Type I-D CRISPR–Cas systems, which are found both in bacteria and archaea, are exceptional in that they contain a hybrid large subunit, Cas10d, bearing resemblance to both the signature proteins found in type I (Cas3) and type III (Cas10). Here, we present the crystal structure of the Cas10d large effector complex subunit from the Sulfolobus islandicus I-D system, both in isolation and in complex with the Sulfolobus islandicus rod-shaped virus 3 (SIRV3) anti-CRISPR protein, AcrID1. As predicted from comparative sequence analysis, the 847 residue (94 kDa) S. islandicus Cas10d consists of six domains: A HD nuclease domain (1–186), a Cyclase/RRM domain (187–425), a zinc finger domain (426–490), a Palm/RRM domain (491–623), and a C-terminal helical region consisting of a polymerase-like Thumb domain (624–719) and an extension with predicted homology to Cas11 (720–847). In this paper, we demonstrate that the S. islandicus type I-D large subunit, Cas10d, has a unique structure consisting of a type I-like HD nuclease domain joined to a set of inactivated type III-like nucleotidyl transferase domains and a Cas11-like C-terminal domain.

To answer this, we finally pursued a structure of the isolated Cas10d subunit. The isolated protein does not readily crystallise likely due to intrinsic flexibility, however, we were able to obtain crystals of a mildly trypsin-treated sample and determine the structure at 4.0 Å using molecular replacement. The new crystals contain two copies of Cas10d in the crystallographic asymmetric unit, for which the flexible N terminus (residues 1–13) that interacts with AcrID1, appears to have been cleaved off. Moreover, the Palm/RRM domain has been nicked by the protease resulting in the protein appearing as two bands on a denaturing polyacrylamide gel. Nevertheless, the structure confirms the overall, extended conformation of Cas10d as observed in complex with AcrID1. The helical insertion in the Palm/RRM domain, which interacts directly with AcrID1 in the complex structure, has shifted away from the core of the protein by about 5 Å in comparison to the complex with AcrID1. Together, this suggests that the flexibility of Cas10d is mainly caused by the extended Palm/RRM domain. Consequently, it is likely that this domain gets organised when Cas10d joins the backbone complex and forms the complete I-D effector complex. In summary, we conclude that the extended structure of Cas10d is an intrinsic feature and not an effect of AcrID1 binding.

>MRNLKRIVMGENKLIGLVRTALDSITLGQGVNEAKIKSPQSYAFHTISVGTISLDICKAIYSSSEIGRKQLENLSKKYNMPFEDLWFYGGFLHDWNKLSGKEESLENKEELTKKIIDKLKLPNEFLHGISTMAEGHLPDNLHLPLWVSIKLADMLLISDIGSVRDVFYFANSDSYRNAIEALKEYNLELNYVSSTFRLFTLIASKELLNDVFNEKSGYFPLISYADGIVFLKRKNSQPVLLSKIVDLLSRQVFSSSSEVIEEKISDIEKCIKNKEELFRQMNIDVKSAIYDEEGKVKQINAFLPTKVCKPFEDVVGNLDNKSKLQVAREVIERNRKDIPFGLLIYFVNKFSKNEEDYIRKGLGINEKSLKYLLNIGDVQKALDKILELLEKRYAEQSSDKTLLYYVKFSSSGNIIDDLPKITDRPNDYCVVCGMPIYSSNPVRFVQYASELGGRAEIWIPREKALDEIDNVRDDWKVCPICIYEANLMKDRVKPPYFIVTFYPGVPISLLNIIDFDFSQSSIKYYIDEEKDTYFTAFEKMGGRLEPYVKKVLPAYFSSKVIIKASEVSNFSLSTRLSKSELNKLLPYAPMISMIFLTSPVLISSNLYEMPIAHERVISITSTYNYTFMKSLNSNLLTLYSIFAYSAKYDAMRKICGRSDLDNCLGYLTEEMDLYSSVDPALGVLSIGMGVGTPIDTDEKFFSAFLPVSGYLLKVTGKVSKMGETLKSSIFSIAYALKDIIKSQKVSKYDVTGFLRDGVDMFFKTTSVIKDKEDRIGISVNAAISSLENKYALDDQHRAQVYSALQDIFKTLYSIEEESDRSLAISIANTLSNWLYIAYKLVLQGDKSLEHHHHHH[2x]> MNNRRKIVVIGASNVGSAVANKIADFQLATEVVLIDLNEDKAWGEA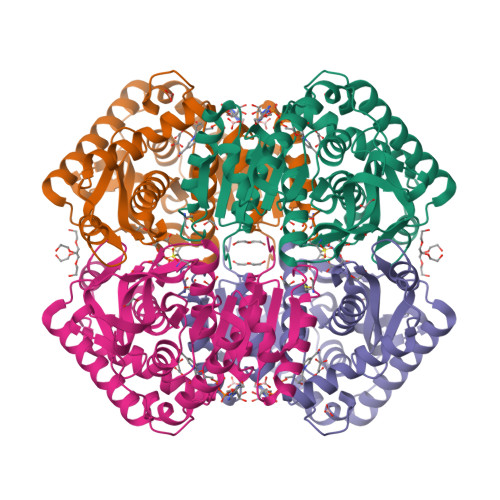KDSSHATSCIYSTNIKFHLGDYEDCKDANIIVITAGPSIRPGETPDRLKLAGTNAKIMSSVMGEIVKRTKEAMIIMITNPLDVATYVVSTQFDYPRNLILGTGTMLETYRFRRILADKYQVDPKNINGYVLGEHGNAAFVAWSTTGCAGFPIDDLDEYFHRTEKLSHEAVEQELVQVAYDVINKKGFTNTGIAMAACRFIKSVLYDEHTILPCSAVLEGEYGIKDVALSIPRMVCADGIMRSFEVHLTDDELEKMHKAAQSVRSALDGAGIKHHHHHH>[2x]SMTVCQLYAKQIRHRGNVKHNTKLG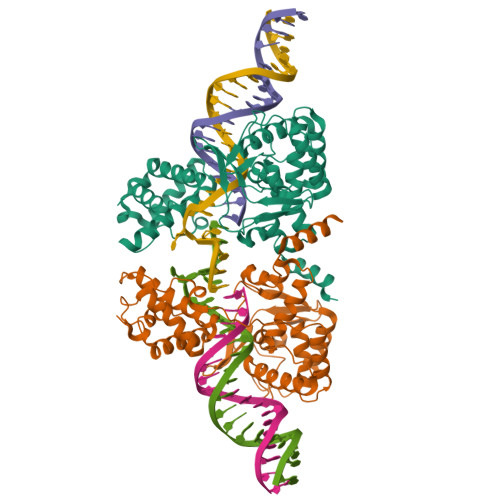RERLMRILEQDRLGSCPIDSVKLSDAKEWALRMKEKGLSYKTINNDKRSLKAAFYTAIQDDCIRKNPFDFQLSDVLDDDTEPKVPLTPAQEESFLSFIQGDKVYQKHYDAIVILLGTGLRISELCGLTDKDLDFENRVIIVSHQLLRNTGVGYYIDEPKTQSGVRKIPMNEEVYQAFQRVIKNRKGAKPFIIDGYANFLFLKQNGYPMTAVDYGGMFGRLVKKYNKSHEEALPKTTTPHAMRHTFCTRLANAGMNPKALQYIMGHSNITMTLNFYAHATFDSARAEMERLAA>KXKVWGSIKR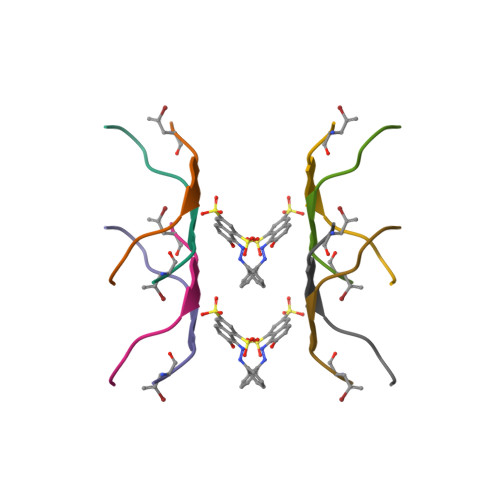L[2x]>[2x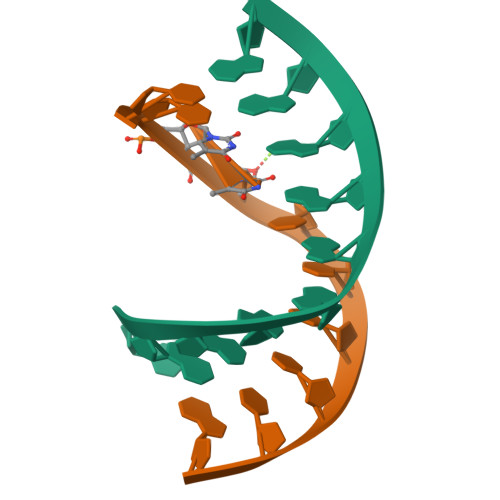]CAAAGAAAAG;>CTXTCTTTG[2x]> MDSSVTNTGGLMPSATISNSEGATMLLNDIPDPTQNVFLSRNVTDNLFEVQDQNLIESLSREVLLGTGTWQSGQAEISTTLTEQQLITNYEQPSIR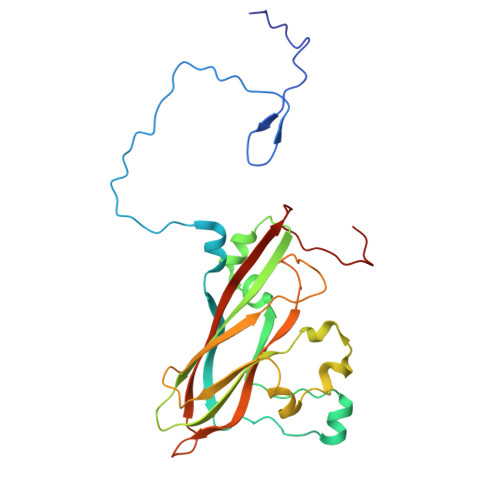QISLPDDIVKGSSFIASKLANIAYMRCDYELYLRVQGSPFLQGLLLLWNKMNADQTSKIRSSITEHLRSITSFPGVTLNMQSDSRSVKLVIPYTSEFQVFNPRNENKLNSVRLSILSALRGPSTSEKATYSIMGRMTNIKLYGHAPSIVSLSYPQTE>[2x]SFQGIRQP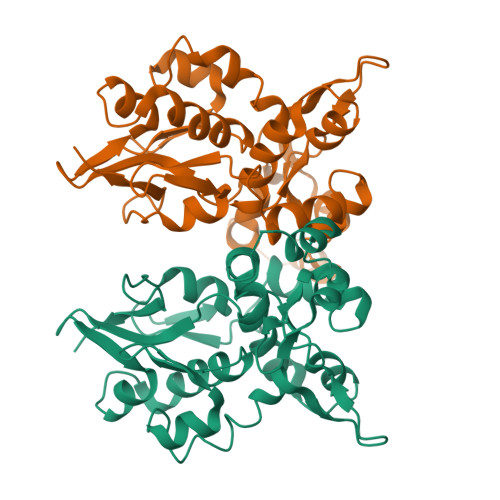VTVTELVDSGILRPSTVNELESGQISYDEVGERIKDFLQGSSCIAGIYNETTKQKLGIYEAMKIGLVRPGTALELLEAQAATGFIVDPVSNLRLPVEEAYKRGLVGIEFKEKLLSAERAVTGYNDPETGNIISLFQAMNKELIEKGHGIRLLEAQIATGGIIDPKESHRLPVDIAYKRGYFNEELSEILSDPSDDTKGFFDPNTEENLTYLQLKERCIKDEETGLCLLPLKEKKKQVQTS>GSTREPEIASSLIKQIFSHYVKTPVTRDAYKIVEKCSERYFKQISSDLEAYSQHAGRKTVEMADVELLMRRQGLVTDKMPLHVLVERHLPLEYRKLLIPIAVSGNKVIPCK[2x];>GRRTVPRGTLRKIIKKHKPHLRLAANTDLLVHLSFLLFLHRLAEEARTNAFENKCKIIKPEHTIAAAKVIL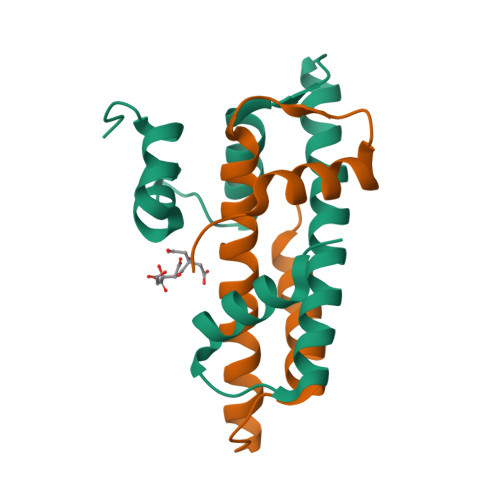KKSRG[2x]>[10x]MAHHHHHHVDDDDKENLYFQGMVAEVQKQAPPFKKTAVVDGIFEEISLEKYKGKYVVLAFVPLAFSFVSPTEIVAF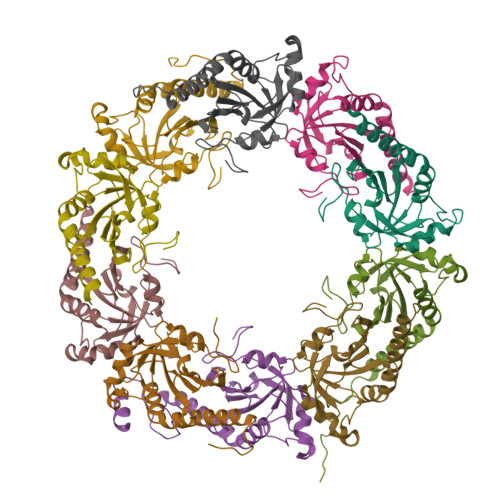SDAAKKFEDQGAQVLFASTDSEYSLLAWTNLPRKDGGLGPVKVPLLADKNHSLSRDYGVLIEKEGIALRGLFIIDPKGIIRHITINDLSVGRNVNEALRLVEGFQWTDKNGTVLPCNWTPGAATIKPDVKDSKEYFKNANN> MTQAKAKHADVPVNLYRPNAPFIGKVISNEPLVKEGGIGIVQHIKFDLTGGNLKYIEGQSIGIIPPGVDKNGKPEQLRLYSIASTRHGDDVDDKTISLCVRQLEYKHPESGETVYGVCSTYLTHIEPGSEVKITGPVGKEMLLPDDPEANVIMLATGTGIAPMRTYLWRMFKDAERAANPEYQFKGFSWLVFGVPTTPNILYKEELEEIQQKYPDNFRLTYAISREQKNPQG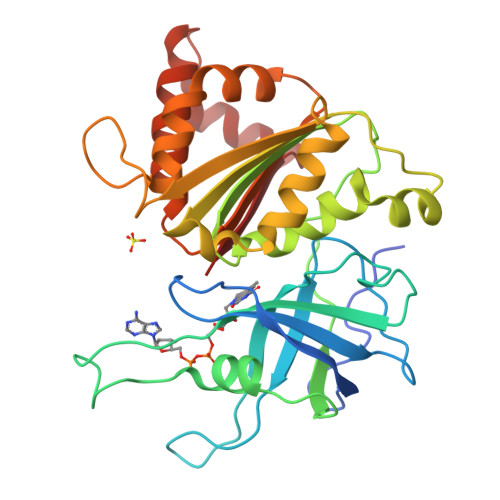GRMYIQDRVAEHADQLWQLIKNQKTHTYICGLRGMEEGIDAALSAAAAKEGVTWSDYQKDLKKAGRWHVETY>L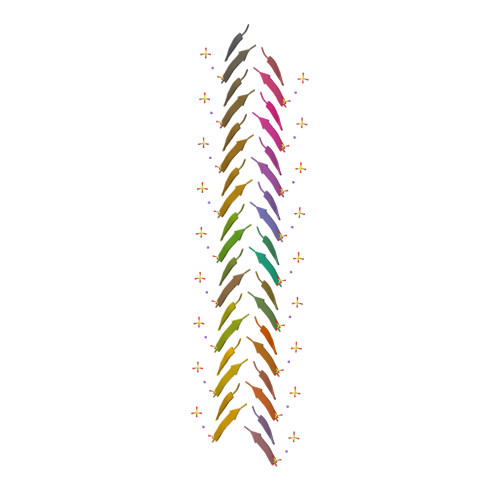FKFFK[2x]>[3x]ASTLKSGSKEVENLKKPFMPPREVHVQVTHSMPPQKIEIFKSLDNWAEENILVHLKPVEKCWQPQDFLPDPASDGFDEQVRELRERAKEIPDDYFVVLVGDMITEEALPTYQTMLNTLDGVRDETGASPTSWAIWTRAWTAEENRHGDLLNKYLYLSGRVDMRQIEKTIQYLIGSGMDPRTENSPYLGFIYTSFQERATFISHGNT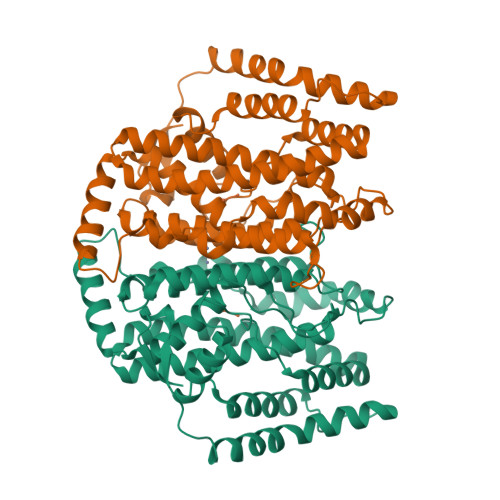ARQAKEHGDIKLAQICGTIAADEKRHETAYTKIVEKLFEIDPDGTVLAFADMMRKKISMPAHLMYDGRDDNLFDHFSAVAQRLGVYTAKDYADILEFLVGRWKVDKLTGLSAEGQKAQDYVCRLPPRIRRLEERAQGRAKEAPTMPFSWIFDRQVKL;> AKKETIDKVSDIVKEKLALGADVVVTADSEFSKLGADSLDTVEIVMNLEEEFGINVDEDKAQDISTIQQAADVIEGLLEKKA>[2x]MTKLITTVKEMQHIVKAAKRSGTTIGFIPTMGALHDGHLTMVRESVSTNDITIVSVFVNPLQFGPNEDFDAYPRQIDKDLELVSEVGADIVFHPAVEDMYPGELGIDVKVGPLADVLEGAKRPGHFDGVVTVVNKLFNIVMPDYAYFGKKDAQQLAIVEQMVKDFNHAVEIIGIDIVREADGLAKSSRNVYLTEQERQEAVHLSKSLLLAQALYQDGERQSKVIIDRV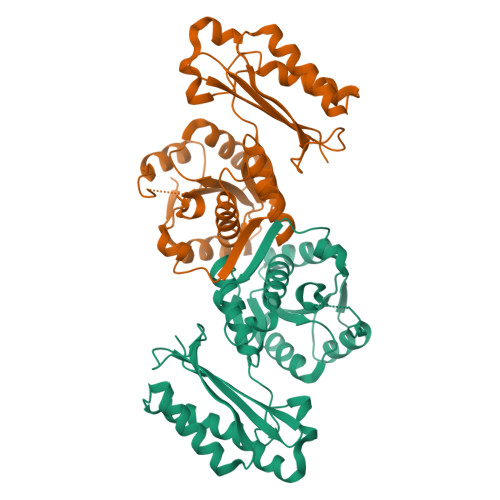TEYLESHISERIEEVAVYSYPQLVEQHEITGRIFISLAVKFSKARLIDNIIIGAE> SASEFNILNDGPPKETYVVDDAGVLSRVTKSDLKKLL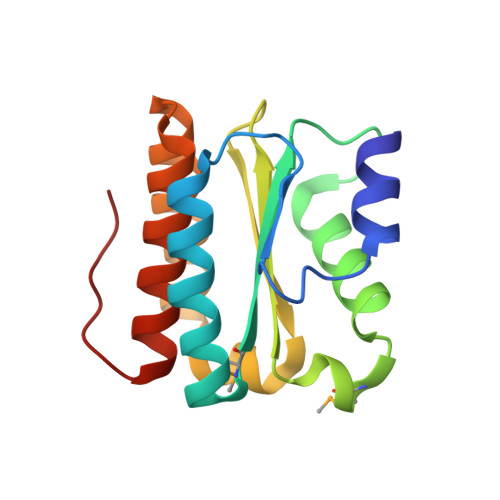SDLEYRKKMRLNFITVRKLTSKADAFEYADQVLEKWYPSMEEGNNKGIVVLITSQKEGAITGGPAFIEAVGENILDATVSENLPVLATDEKYNEAVYSSAKRLVAAIDGQPDPGGP>[8x]MHHHHHHHHHHLEVLFQGPSEFPMAQSNIIAGMDLNRLDRIAEHLDRAYLHPGKLAGTMTLVARRGEVVYCQAQGLRDV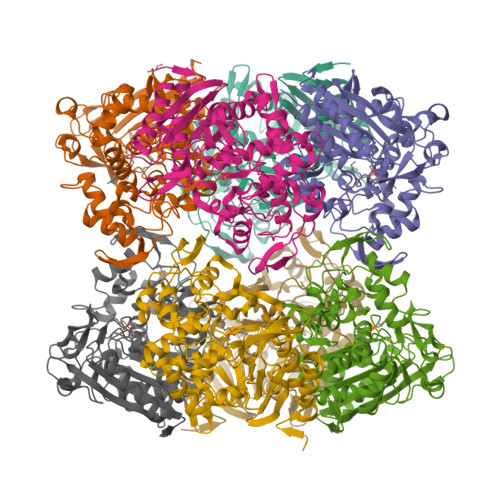ERQLPVERDTLFRIYSMTKPITSIALMQLYEQGRFLLDEPVHKYIPTWKNLRVYKTGSHPQMLTTAPQRPMTIRDLLTHQSGLTYGFMNRTNVDAAYRSLKLDGGPGHTLDRLIDELARLPLEFSPGTAWNYSVATDVCGYLVQLLSGMSLDDYFSKHIFQPLGMPDTFFTVPAEKLSRFAACYEYQPGDSFSLQDDPQGSAFAKAHGYLSGGGGLVSCVDDYYRFAQALANGGELDGARIIGRKTLEFMRMNHLPDNKGLPDVAIGSFSETPYDGTGFGLGFSVKLDVAKSQTVGSVGEYGWGGMASTNFFIDPEEDLLMVFMTQLIPSSTYAVRQELRAIINGALVDA>[2x]TNLRVLLDTAIPPSFCDTVSSVLLDDFNMVSLIRTSPADSLATIKQDNAEIDIAITIDEELKISRFNQCVLG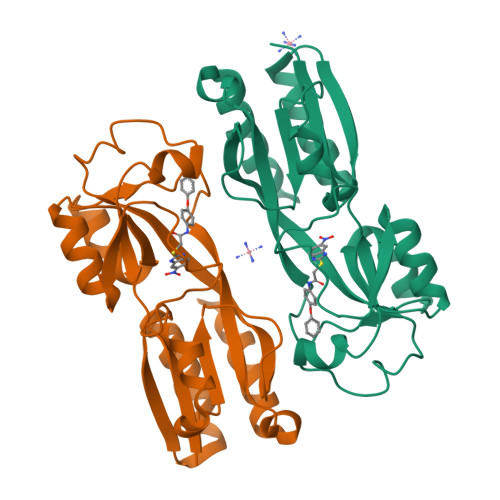YTKAFVVAHPQHPLCNASLHSIASLANYRQISLGSRSGQHSNLLRPVSDKVLFVENFDDMLRLVEAGVGWGIAPHYFVEERLRNGTLAVLSELYEPGGIDTKVYCYYNTALESERSFLRFLESARQRLREL> MHHHHHHMNFNVSLMEKLKWKIKCIENKFLNYRLTTNETVVAETEYGKVKGVKRL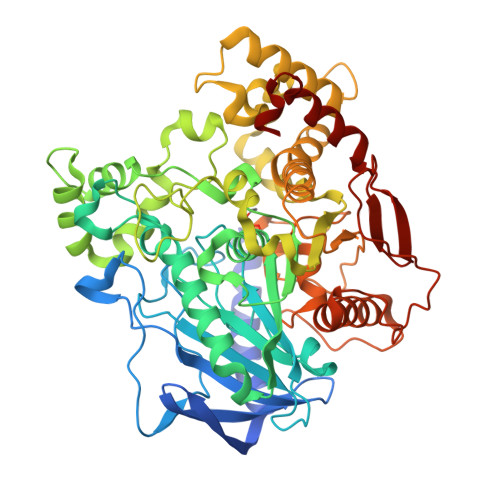TVYDDSYYSFEGIPYAQPPVGELRFKAPQRPTPWDGVRDCCNHKDKSVQVDFITGKVCGSEDCLYLSVYTNNLNPETKRPVLVYIHGGGFIIGENHRDMYGPDYFIKKDVVLINIQYRLGALGFLSLNSEDLNVPGNAGLKDQVMALRWIKNNCANFGGNPDNITVFGESAGAASTHYMMLTEQTRGLFHRGILMSGNAICPWANTQCQHRAFTLAKLAGYKGEDNDKDVLEFLMKAKPQDLIKLEEKVLTLEERTNKVMFPFGPTVEPYQTADCVLPKHPREMVKTAWGNSIPTMMGNTSYEGLFFTSILKQMPLLVKELETCVNFVPSELADAERTAPETLEMGAKIKKAHVTGETPTADNFMDLCSHFYFWFPMHRLLQLRFNHTSGTPVYLYRFDFDSEDLINPYRIMRSGRGVKGVSHTDELTYFFWNQLAKRMPKESREYKTIERMTGIWTQFATTGNPYSNEIEGMENVSWDPIEKSDEVYKCLNISDELKMIDVPEMGKIKQWESMFEKHRDLF> MSSGLRAADFPRWKRHISEQLRRR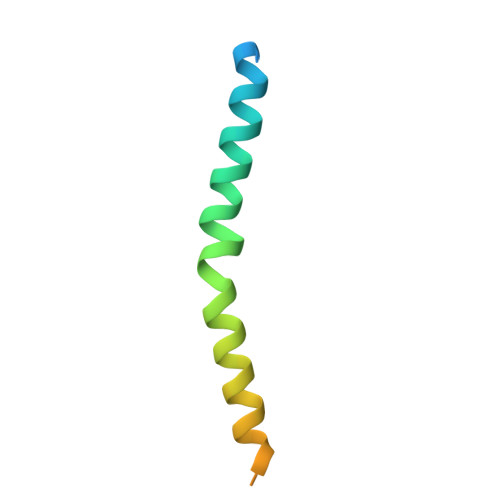DRLQRQAFEEIILQYNKLLEKSDLHSVLAQKLQAEKHDVPNRHEI> TQVLNGYWGYQEFLDEFPEQRNLTNALSEAVRAQPVPLSKPTQRPIKISVVYPGQQV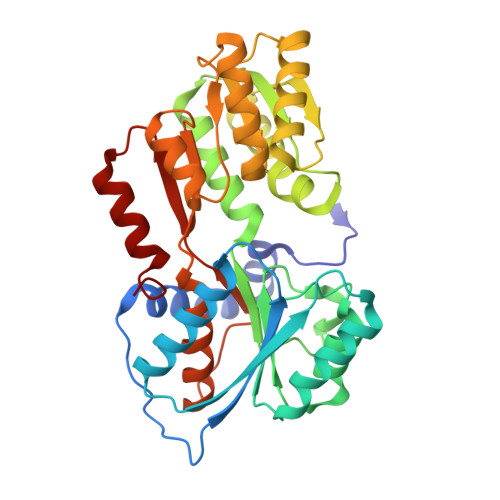SDYWVRNIASFEKRLYKLNINYQLNQVFTRPNADIKQQSLSLMEALKSKSDYLIFTLDTTRHRKFVEHVLDSTNTKLILQNITTPVREWDKHQPFLYVGFDHAEGSRELATEFGKFFPKHTYYSVLYFSEGYISDVRGDTFIHQVNRDNNFELQSAYYTKATKQSGYDAAKASLAKHPDVDFIYACSTDVALGAVDALAELGREDIMINGWGGGSAELDAIQKGDLDITVMRMNDDTGIAMAEAIKWDLEDKPVPTVYSGDFEIVTKADSPERIEALKKRAFRYSDN Subsequent studies in C. elegans, Xenopus, Zebrafish, and Drosophila confirmed the role of UNC-45 as a myosin-specific chaperone, promoting the folding of the myosin ATPase domain as well as coordinating the assembly of thick filaments during muscle development. To better understand its myosin folding function, we established an orthogonal protein folding assay in insect cells, characterizing the interplay of the C. elegans muscle myosin MHC-B with its cognate chaperone UNC-45. Structural data of various functional mutants clarify the role of the distinct UNC-45 domains in this process providing important mechanistic insight into its myosin folding activity.

In contrast, none of the ts-proteins shifted into the HMW fraction further confirming that the ts-mutants, present in a folded state, cannot interact with damaged myosin. Together, the cellular folding assay, the CD data and the SEC-based reconstitution analysis demonstrate that the ts-mutations L559S, G427E, E781K and L822F have a direct effect on the myosin-binding function of UNC-45, abrogating the interaction with the heat-damaged myosin substrate. To address the structural basis of the impaired chaperone function of UNC-45 ts-mutants L822F and G427E, and UNC-45 ΔTPR, we analyzed the crystal structures of the three mutant proteins. The two UNC-45 ts-mutants L822F and G427E crystallized in the form of a linear filament, having the same periodicity (85 Å), hydrophobic interface and overall domain organization as the previously characterized wt oligomer. However, when we compared the UCS domains of wt and ts UNC-45, we noted two major differences. First, the ts UCS domains adopt different conformations, as most clearly seen for the C-terminal portion of the UCS domain that moves about 10–15 Å. Moreover, as revealed by the L822F structure, the entire UCS domain is able to move en-bloc towards the TPR/central domain backbone of the UNC-45 molecule. A second difference of wt UNC-45 and ts mutants comprises the dynamics of the UCS domain. In contrast, the two ts mutants crystallized exclusively in one state, even when testing a large number of crystals for an alternate crystal form. Likewise, the L822F ts mutation causes local changes inducing movement of the UCS domain towards the TPR/central backbone. As for the G427E mutant, the established inter-domain contacts reduce the conformational flexibility of the UCS domain, which seems to be a common property of the analyzed ts mutants.

> MVARVQTAEEIRDEGNAAVKDQDYIKADELYTEALQLTTDEDKALRPVLYRNRAMARLKRDDFEGAQSDCTKALEFDGADVKALFRRSLAREQLGNVGPAFQDAKEALRLSPNDKGIVEVLQRLVKANNDKIKQTTSLANKVTDMEKLAFRGEAKDTEQKMTALNNLLVLCRESESGATGVWNQGALVPFVLNLINDASENEEVTVTAIRILDETIKNSVRCMKFLAMHDPDGPKSVRFVCRLMCKKSTKDFVDATGILVQRVFNAMAKMDRQKEMKPDPEVAEANKIWIIRVLLELQEMLQDPKVGAVQRETCIDLFLKNLMHMDGGIPRGWSWKFVEERGLLALLDVASQIPELCEYPVSAETRQHVAICLQRLEEDMVFDTKRTIFKEKVDMFFNALISRCTNDDEGHKYRIKLSCFLITMLQGPVDIGINLITNDQLTPIMLEMAASQDHLMQGIAAELIVATVSKHERAINMLKVGIPVLRALYDSEDPTVKVRALVGLCKIGAAGGDDISKATMKEEAVISLAKTCKKFLLETEKYSVDIRRYACEGLSYLSLDADVKEWIVDDSLLLKALVLLAKKAGALCVYTLATIYANLSNAFEKPKVDEEMVKLAQFAKHHVPETHPKDTEEYVEKRVRALVEEGAVPACVAVSKTESKNALELIARSLLAFAEYEDLRGRIIAEGGTVLCLRLTKEASGEGKIKAGHAIAKLGAKADPMISFPGQRAYEVVKPLCDLLHPDVEGKANYDSLLTLTNLASVSDSIRGRILKEKAIPKIEEFWFMTDHEHLRAAAAELLLNLLFFEKFYEETVAPGTDRLKFWVLYSAEVEEERLSRASAAGFAILTEDENACARIMDEIKSWPEVFKDIAMHEDAETQRRGLMGIANIMHSSNKLCSEIVSSEVFRVLVAVTKLGTINQERAGSTEQAKRGLEAAEKFGLIKATDREIYERENQMSTIQE>[4x]MNVVVIGGGAAGLKAASRIRRKDGDASITVVEAGKYVSLGRCGLPYYVGGLVHEVDNLRETTYGAVRDEAYFKKLKNIDVLTETVATEIDRSRKTVKIVRNGSEDELNYDYLVIATGARPAKPPIEGIEAEGVVTLTSAEEAEKIIEMWEEGAEKAVVIGAGFIGLESAEALKNLDMEVTVIEMMDRVAPAMLDREMAVLVENHLREKGVNVVTSTRVEKIVSQDDKVRAVIANGKEYPADVVVVATGIKPNSELAEKAG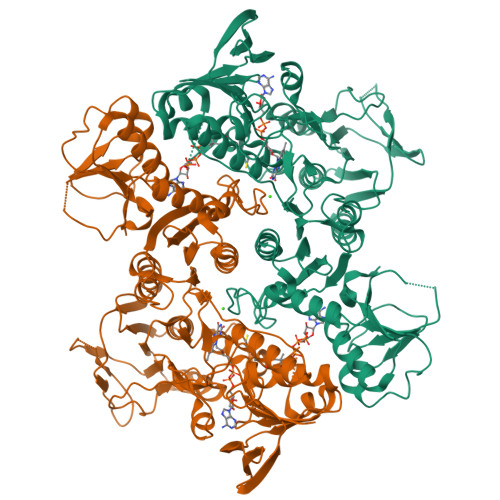LKIGETGAIWVDEYMRTSDESIYAGGDCVETTCLVTGKKIIAPFGDVANKQGRVIGENITGGRAVFPGVIRTAIFKVFDFTAASAGVNEQMAKEAGLDYFTVIAPSPDRAHYYPQANYIRLKLIVEKGSWRVIGAQGVGMGEVAKRIDVLSTAIQAGMTIDQLANLDLAYAPPYSPALDPVITIANVAMNKRDGLFEGINVFELKEKLEKEDIVILDVRSEEEFKTRRIESEKVIHIPILELRERLDEIPRDKEIVVVCAIGLRSFEASRILKHAGFEKVKILEGGMAFWF> HMCNKNNTFEKNLDISHKPEPLILFNKDNNIWNSKYFRIPNIQLLNDGTILTFSDIRYNGPDDHAYIDIASARSTDFGKTWSYDIAMKNNRIDSTYSRVMDSTTVITNTGRIILIAGSWNTNGNWAMTTSTRRSDWSVQMIYSDDNGLTWSNKIDLTKDSSKVKNQPSNTIGWLGGVGSGIVMDDGTIVMPAQISLRENNENNYYSLIIYSKDNGETWTMGNKVPNSNTSENMVIELDGALIMSTRYDYSGY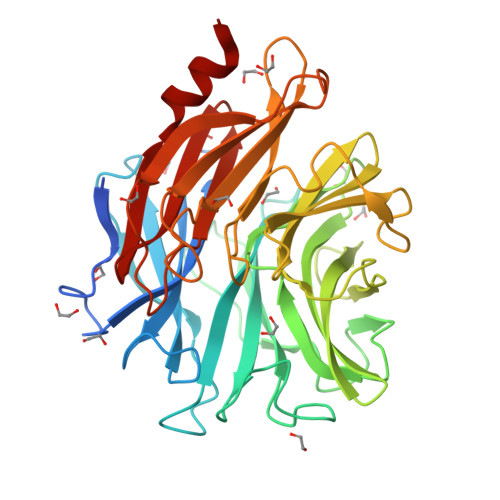RAAYISHDLGSTWEIYEPLNGKVLTGKGSGCQGSFIKATTSNGHRIGLISAPKNTKGEYIRDNIAVYMIDFDDLSKRVQEICIPYPKDGNKLGGGYSCLSFKNSHLSIVYEANGNIEYQDLTPYYSLINKQ> MRGSHHHHHHGSDPAPDAVAQQWAIFRAKYLRPSGRVVDTGNGGESHSEGQGYGMLFAASAGDLASFQSMWMWARTNLQHTNDKLFSWRFLKGHQPPVPDKNNATDGDLLIALALGRAGKRFQRPDYIQDAMAIYGDVLNLMTMKAGPYVVLMPGAVGFTKKDSVILNLSYYVMPSLLQAFDLTADPRWRQVMEDGIRLVSAGRFGQWRLPPDWLAVNRATGALSIASGWPPRFSYD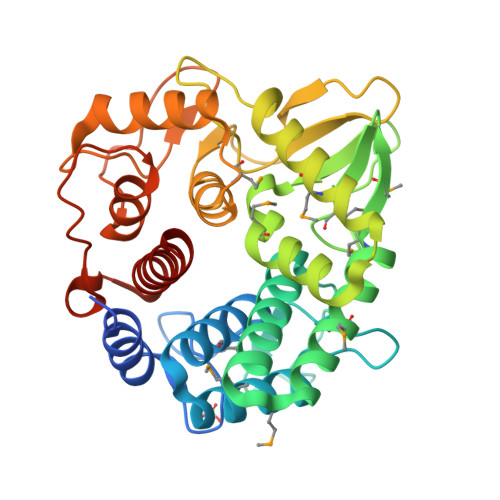AIRVPLYFYWAHMLAPNVLADFTRFWNNFGANALPGWVDLTTGARSPYNAPPGYLAVAECTGLDSAGELPTLDHAPDYYSAALTLLVYIARAEETIK>MSPFPLTSMDKAFITVLEMTPVLGTEIINYRDGMGRVLAQDVYAKDNLPPFPASVKDGYAVRAADGPGDRFIIGESQAGEQPTQTVMPGQVMRVTTGAPIPCGADAVVQVEDTELIRESDDGTEELEVRILVQARPGQDIRPIGHDIKRGECVLAKGTHMGPSEIGLLATVGVTEVEVNKFPVVAVMSTGNELLNPEDDLLPGKIRDSNRSTLLATIQEHGYPTINLGIVGDNPDDLLNALNEGISRADVIITSGGVSMGEKDYLKQVLDIDLHAQIHFGRVFMKPGLPTTFATLDIDGVRKIIFALPGNPVSAVVTCNLFVVPALRKMQGILDPRPTIIKARLSCDVKLDPR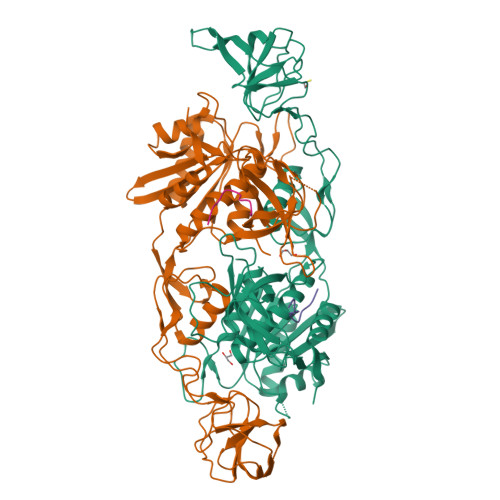PEYHRCILTWHHQEPLPWAQSTGNQMSSRLMSMRSANGLLMLPPKTEQYVELHKGEVVDVMVIGRL[2x];>FNIVGTTYPIN[2x]> MMAPANNPFGAPPAQVNNP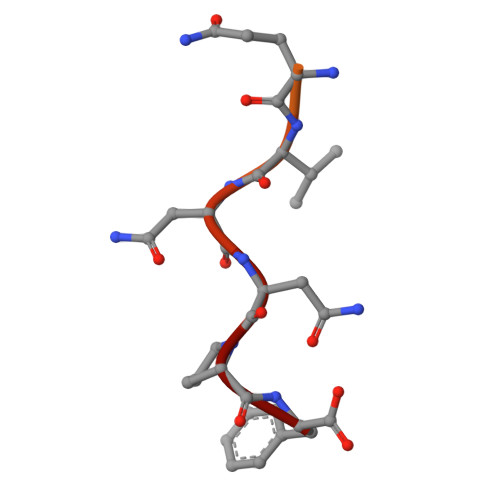F>[4x]MDYTKYLAGRANWIKGSALADVMKKASELQKKGVKLISLAAGDPDPELIPRAVLGEIAKEVLEKEPKSVMYTPANGIPELREELAAFLKKYDHLEVSPENIVITIGGTGALDLLGRVLIDPGDVVITENPSYINTLLAFEQLGAKIEGVPVDNDGMRVDLLEEKIKELKAKGQKVKLIYTIPTGQNPMGVTMSMERRKALL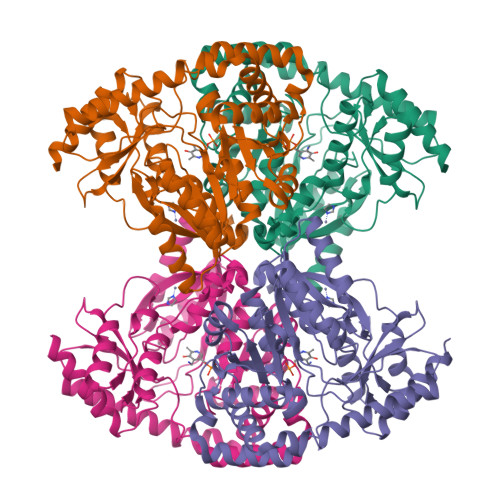EIASKYDLLIIEDTAYNFMRYEGGDIVPLKALDNEGRVIVAGTLSKVLGTGFRIGWIIAEGEILKKVLMQKQPIDFCAPAISQYIALEYLKRGYFEKYHLEGALLGYKEKRDIMLKALENHLPNAEFTKPIAGMFVMFFLPEGADGISFANELMEREGVVVVPGKPFYTDESGKNAIRLNFSRPSKEEIPIGIKKLAKLYKEKFGE>GAMGPQEYTLIKLKIHLIPEFLGSIVKGREVFVVCATLRPETMYGQTNCWILPDGEYDLVLAFDQVIPYDAKTSDGVLCKIFDKYEDTMKECNTVYICSERSAYNMAYQGIVPLIHGREQGVSDKLLPRIVSLGKVYGEQLIGTPLSAPMTPYSLIFILPMFSISMEKGTGIVTSVPSDSPDDYAALRDIKTKPLLREKYSIKDEWILDPLEIIEVPGFGFMTAELLCNQYKIQSQNDSAKLKQAKEEIYKKEFYEGILIRGKYSGMKICDAKELIRESLIKDGYALIYLE[3x];> GAMGPQEYTLIKLKIHLIPEFLGSIVKGREVFVVCATLRPETMYGQTNCWILPDGEYDLVLAFDQVIPYDAKTSEGVLCKIFDKYEDTMKECNTVYICSERSAYNMAYQGIVPLIHGREQGVSDKLLPRIVSLGKVYGEQLIGTPLSAPMTPYSLIFILPMFSISMEKGTGIVTSVPSDSPDDYAALRDIKTKPLLREKYSIKDEWILDPLEIIEVPGFGFMTAELLCNQYKIQSQNDSAKLKQAKEEIYKKEFYEGILIRGKYSGM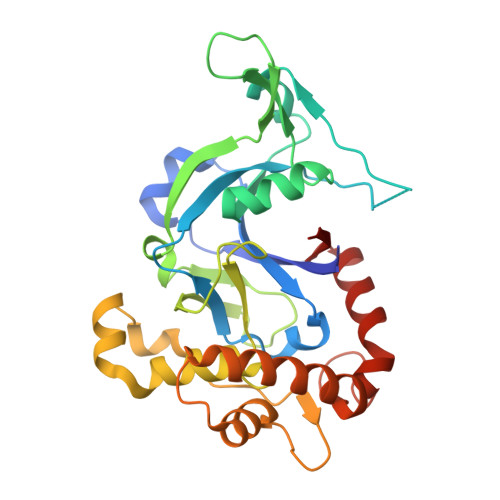KICDAKELIRESLIKDGYALIYLE GK catalyses the rate-limiting step of glycerol utilization, with phosphorylation serving to sequester the sugar in the cell. The 501-residue GK polypeptide is arranged as two domains separated by a deep cleft. Each domain is constructed around a βββαβαβα core that is characteristic of the sugar kinase/Hsp70/actin superfamily of proteins. In agreement with gel filtration experiments (data not shown), PfGK is a dimer in the crystal.

The PfGK–ADP crystals have different cell parameters and it is apparent that domains I and II have moved apart and that the enzyme is in an ‘open’ conformation. The relative domain movement can be described as a 27.5° rotation, substantially larger than the 7° rotation deduced from crystal structures of orthologous enzymes. In the dimer, the long axis increases in length from 97 Å to 117 Å, exposing a further 1500 Å2 of solvent accessible surface area around the active site. In the open (ADP-bound) structure, interdomain contacts such as Gln12-Thr268 and the salt-bridges Arg83-Glu306 and Glu109-Arg363 are ruptured. Aspects of the glycerol pocket are maintained, with a pair of ethylene glycol (cryoprotectant) molecules clearly mimicking protein interactions formed by glycerol. However, as a result of domain movement, Phe271 and Tyr135 are significantly displaced. In contrast to glycerol, which binds predominantly to domain I, ADP in the PfGK–ADP complex is bound exclusively to domain II. ADP is bound with the adenine base tucked into a pocket and the ribose and phosphate moieties more exposed on the enzyme surface extending towards the interdomain cleft. The adenine base forms polar interactions with Asn418 and Ser332. The rather modest set of polar interactions with the ribose and phosphate groups involving Thr268, Gly313, Gly414 and Met415 are likely to be augmented in the ternary closed complex with ATP.

>[2x]ISEFGSMNVILSIDQSTQSTKVFFYDEELNIVHSNNLNHEQKCLKPGWYEHDPIEIMTNLYNLMNEGIKVLKDKYTSVIIKCIGITNQRETVIIWDRITGKPLYNAIVWLDTRVEELVTEFSAKYNNNDIQKKTGTYFNTYFSAFKILWLIQNNPEIKQKIDDGTAVIGNINTWLIFNLTKGNCYTDVTNASRTLLMDINTLQWDEKMCKIFNITNMSVLPEIKSNCSNFGLVKSEHVPDYLNIPITGCIGDQQSACIGQAIFDEGEAKCTYGTGVFLLINTGEKVVYSTCGLITTICYKFNDNDKPKYALEGSIGTAGSGVSWLLKNKLIDDPSEASDIMEKCENTTGVIFVPAFSGLYAPRWRSDARASIYGMTFNTERSHIVRALLEGIAFQLNEIVDSLTSDMGIEMLHVLRCDGGMTKNKPFMQFNSDIINTKIEVSKYKEVTSLGAAVLAGLEVKIWDSLDSVKSLLRRSDAVFHSKMDDKKRKKKTSEWNKAVERTLIQL>[8x]ADQPIDADVTVIGSGPGGYVAAIKAAQLGFKTVCIEKNETLGGTCLNVGCIPSKALLNNSHYYHMAHGTDFASRGIEMSEVRLNLDKMMEQKSTAVKALTGGIAHLFKQNKVVHVNGYGKITGKNQVTATKADGGTQVIDTKNILIAT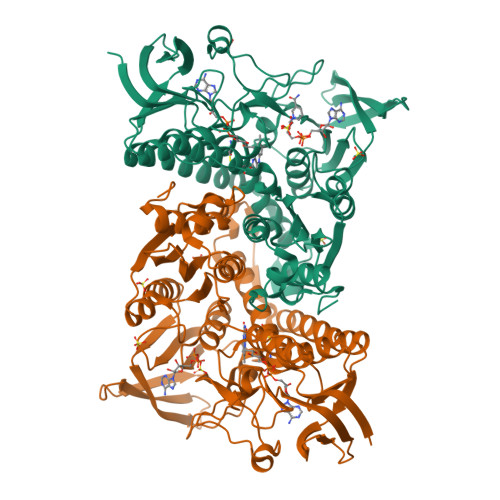GSEVTPFPGITIDEDTIVSSTGALSLKKVPEKMVVIGAGVIGVELGSVWQRLGADVTAVEFLGHVGGVGIDMEISKNFQRILQKQGFKFKLNTKVTGATKKSDGKIDVSIEAASGGKAEVITCDVLLVCIGRRPFTKNLGLEELGIELDPRGRIPVNTRFQTKIPNIYAIGDVVAGPMLAHKAEDEGIICVEGMAGGAVHIDYNCVPSVIYTHPEVAWVGKSEEQLKEEGIEYKVGKFPFAANSRAKTNADTDGMVKILGQKSTDRVLGAHILGPGAGEMVNEAALALEYGASCEDIARVCHAHPTLSEAFREANLAASFGKSINF> MVQAWYMDESTADPRKPHRAQPDRPVSLEQLRTLGVLYWKLDADKYENDPELEKIRKMRNYSWMDIITICKDT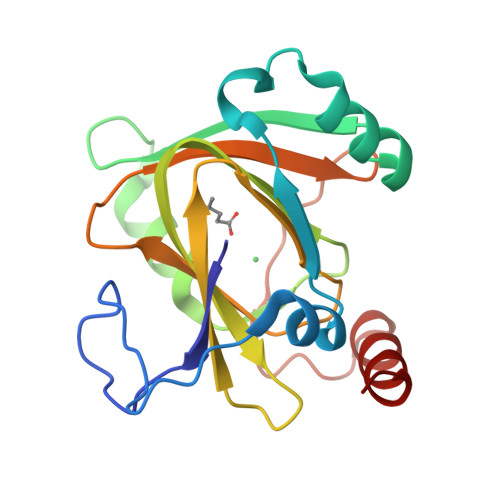LPNYEEKIKMFFEEHLHLDEEIRYILEGSGYFDVRDKEDKWIRISMEKGDMITLPAGIYHRFTLDEKNYVKAMRLFVGEPVWTPYNRPADHFDARVQYMSFLEGTA1-[(3-hydroxyphenyl)methyl]-3-(4-pyridin-4-yl-1,3-thiazol-2-yl)urea 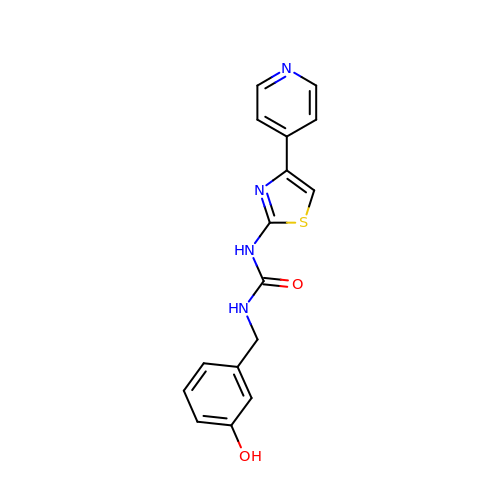| C16 H14 N4 O2 S | GDVRVPIXWXOKQO-UHFFFAOYSA-N PHOSPHONOACETALDEHYDE | C2 H5 O4 P | 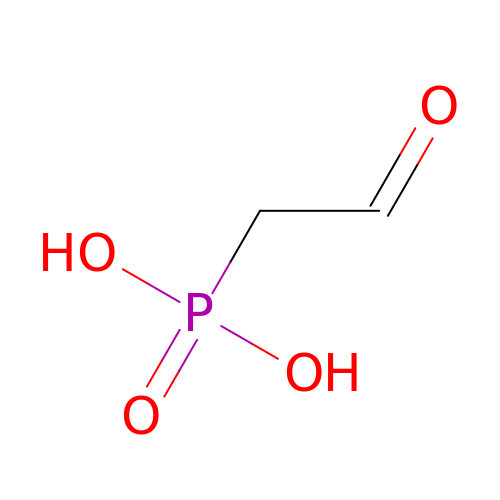YEMKIGUKNDOZEG-UHFFFAOYSA-N>[2x]MMFNFYQFLYNLQNVSPFIDFSVLKQLTHTKMRENEPARFETRSFSQLIDHARSWKTEVRGMTTQGFTKISLMRAEKDRLNMYAISSVPGTNTQSIFSVTIPLELVEKAQVADRKFELKLKSGYNVDSYIRKTPPSAEFTLQCERQRSQVVTGISDYEIRNGKMILMAGDQLFRYNPLNEALAAIPIAVPDDQSSTEPMDISEGSITSGTKGSGSEAPQSSTVPPVTRIPIKKPTTSTEKPATAPPTNNFVSSAKVCPADSSLLAYVLNKQVYIEKNGKIIHRTSSNSKHITNGVPSYIVQEELERFEGIWWSESKTRLLYEHVNEEKVAESQFGVNGDPPVAPMKYPRAGTKNAYSTLRMVILENGKAYDVPLKDEVIYKHCPFYEYITRAGFFSDGTTVWVQVMSRDQAQCSLLLIPYTDFLLPEELGGSIKEDNLQLSTDLNMGVWDDKSHEETMEKPPRGKLRGTVQIHKARNDYWINTHNAIYPLKITDEEHPMYEFIYCLEKPNGSCLALISAELDQNGYCRHTEEKLLMAENFSINKSMGIVVDEVRELVYYVANESHPTEWNICVSHYRTGQHAQLTESGICFKSERANGKLALDLDHGFACYMTSVGSPAECRFYSFRWKENEVLPSTVYAANITVSGHPGQPDLHFDSPEMIEFQSKKTGLMHYAMILRPSNFDPYKKYPVFHYVYGGPGIQIVHNDFSWIQYIRFCRLGYVVVFIDNRGSAHRGIEFERHIHKKMGTVEVEDQVEGLQMLAERTGGFMDMSRVVVHGWSYGGYMALQMIAKHPNIYRAAIAGGAVSDWRLYDTAYTERYMGYPLEEHVYGASSITGLVEKLPDEPNRLMLVHGLMDENVHFAHLTHLVDECIKKGKWHELVIFPNERHGVRNNDASIYLDARMMYFAQQAIQGFGPTTAAPRQGPLWSHPQFEK

To examine the substrate specificity of a second DPP-IV family exopeptidase, we selected C. elegans DPF-3, a DPP8/9-orthologue that promotes male fertility through N-terminal processing of two large RNA-binding proteins, WAGO-1 and WAGO-3. The overall structure follows the conserved dipeptidyl peptidase (DPP) fold that is characterized by two domains, a C-terminal hydrolase with α/β fold, and an N-terminal β-propeller domain encompassing eight blades as observed in other DPPIVs. We validate the specificity of the motifs through applying qPISA to another member of the DPP-IV family, C. elegans DPF-3, an orthologue of human DPP8/9, which reveals a related but distinct cleavage motif. Through a DPF-3 structure that we solve using cryogenic electron microscopy (cryo-EM), we can rationalize differences in the subsite interactions between the two exopeptidases.

To relate the observed differences in substrate specificities of DPF-3 and DPP4 to structure, we determined the structure of DPF-3 to an effective resolution of 2.6 Å by single particle cryogenic Electron Microscopy (cryo-EM). The map was interpretable for residues 37–123, 259–431, and 470–916. DPF-3 superposes with the apo structures of its orthologues DPP8 and DPP9 with r.m.s.d. A comparison of the DPF-3 apo structure with DPP4 reveals an S1 subsite that is nearly identical for both enzymes, with all amino acids being conserved. Instead, the divergent enzymatic footprints appear best explained by differences in the S2 and S1’ subsites. Unlike DPP4, DPF-3 contains an acidic residue (E309) but lacks a bulged loop inserting a hydrophobic/aromatic residue (F357 in DPP4) into the S2 subsite, which alters its geometry and chemical environment substantially. E309, which structurally aligns with a serine in DPP4 (S209), is adjacent to the double glutamate motif that is required to position the terminal NH3+ group. Another significant difference from DPP4 is the presence of an isoleucine (I705) in the S1’ subsite of DPF-3 that is oriented towards the P1’ substrate position. In DPP4, the corresponding side chain is a serine (S552), which is retracted from the substrate along with a segment of the loop. This difference is consistent with DPF-3’s enhanced preference for several hydrophobic and all aromatic amino acids at P1’, because the isoleucine may facilitate hydrophobic packing of these side chains to contribute to substrate binding or positioning.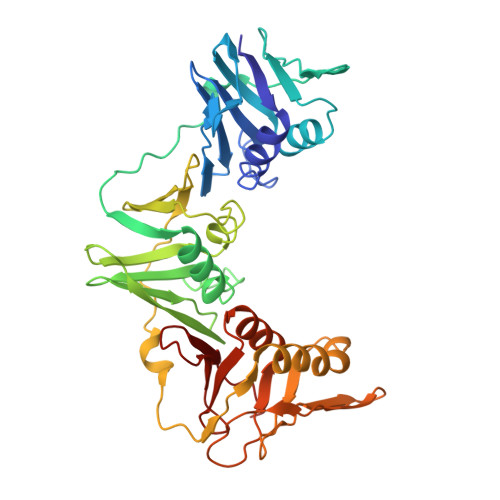> MMEFTIKRDYFITQLNDTLKAISPRTTLPILTGIKIDAKEHEVILTGSDSEISIEITIPKTVDGEDIVNISETGSVVLPGRFFVDIIKKLPGKDVKLSTNEQFQTLITSGHSEFNLSGLDPDQYPLLPQVSRDDAIQLSVKVLKNVIAQTNFAVSTSETRPVLTGVNWLIQENELICTATDSHRLAVRKLQLEDVSENKNVIIPGKALAELNKIMSDNEEDIDIFFASNQVLFKVGNVNFISRLLEGHYPDTTRLFPENYEIKLSIDNGEFYHAIDRASLLAREGGNNVIKLSTGDDVVELSSTSPEIGTVKEEVDANDVEGGSLKISFNSKYMMDALKAIDNDEVEVEFFGTMKPFILKPKGDDSVTQLILPIRTY2-(4'-AMIDINOBIPHENYL-4-YL)-1H-BENZIMIDAZOLE-5-AMIDINE 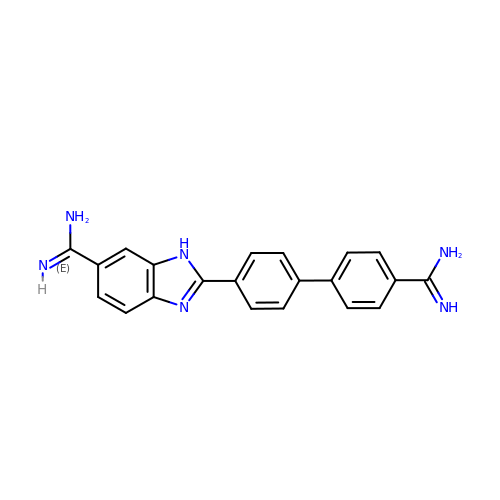| C21 H18 N6 | MIMVUHYHAXPADM-UHFFFAOYSA-N>MKTAALFVSKEFEEEAIALVEGANYKVTSIYKLPKSPNVKFYIQYDKLQQIKNDEEISTLIIFEQLKPRHFINIRRELKGKEVLDKILLLLEIFALHAGSKEAKMQIELARLKYELPIIKETYTKSKIGEQQGPLGAGTYGVESTIKFYKRRINKLMKELESIKIFKEKSIESNKRNNIPSIGIVGYTNSGKTSLFNSLTGLTQKVDTKLFTTMSPKRYAIPINNRKIMLVDTVSFIRGIPPQIVDAFFVTLSEAKYSDALILVIDSTFSE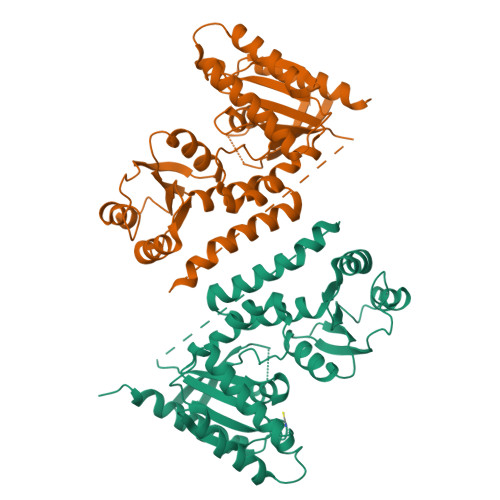NLLIETLQSSFEILREIGVSGKPILVTLNKIDKINGDLYKKLDLVEKLSKELYSPIFDVIPISALKRTNLELLRDKIYQLATQLSLEHHHHHH[2x]> MFKHKHPFGGAFLPEELLAPIQNLKAEWEILKTQQSFLSELDCILKNYAGRQTPLTEVKNFARAIDGPRVFLKREDLLHTGAHKLNNALGQCLLAKYLGKTRVVAETGAGQHGVATATACAYLGLDCVVYMGAKDVERQKPNVEKMRFLGAEVVSVTKGSCGLKDAVNQALQDWATTHSFTHYCLGSALGPLPYPDIVRFFQSVISAEVKEQIHAVAGRDPDILIACIGGGSNAIGFFHHFIPNPKVQLIGVEGGGLGISSGKHAARFATGRPGVFHGFYSYLLQDDDGQVLQTHSISAGLDYPSVGPDHAEMHESGRAFYTLATDEEALRAFFLLTRNEGIIPALESSHALAHLVSIAPSLPKE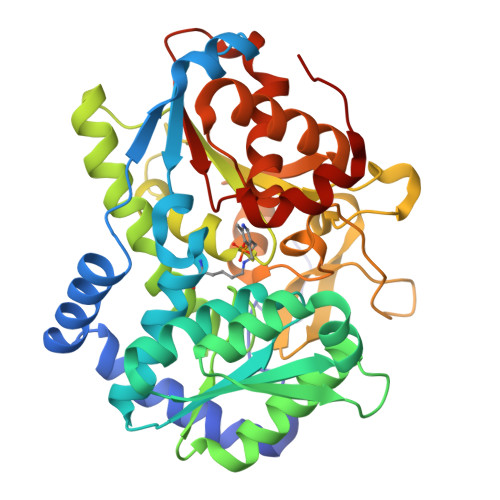QIVIVNLSGRGDKDLPQIIRRNRGIYE>[2x]MSLALYLGNKRMNDMYYTIGQVAKMQHLTISQIRYYDKQGLFPFLQRNEKGDRIFNEEALKYLEMILCLKNTGMPIQKIKQFIDW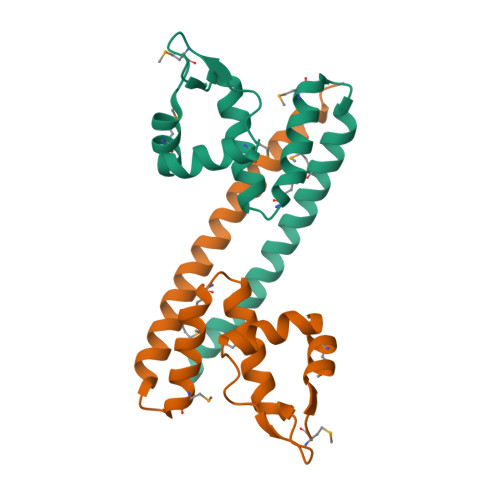SMEGDSTILHRLKLMKQQEANVLQLIQDTEKNLKKIQQKIAKYEDEISSANATTKEGHHHHHH5'-O-[(S)-{[(R)-(2-aminoethyl)(hydroxy)phosphoryl]oxy}(hydroxy)phosphoryl]cytidine | C11 H20 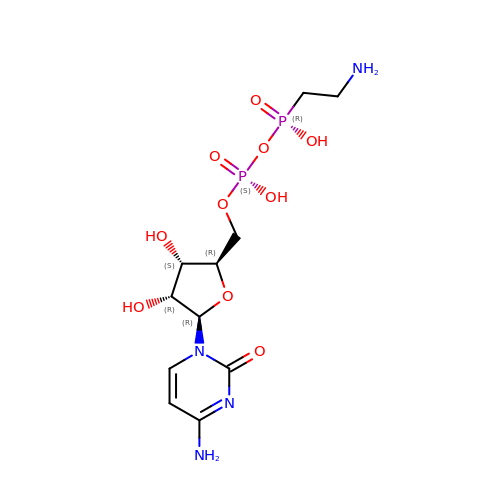N4 O10 P2 | FBADRUOBFLBKJQ-PEBGCTIMSA-N> QVTPRPEAAPGARPGFRAPARIISPEIMPDNKVTFRVYSKDASKVTITGEWQTGPGGVEELVKNDTGMFSITVGPLKPELYAYNFTVDGVKALDANNV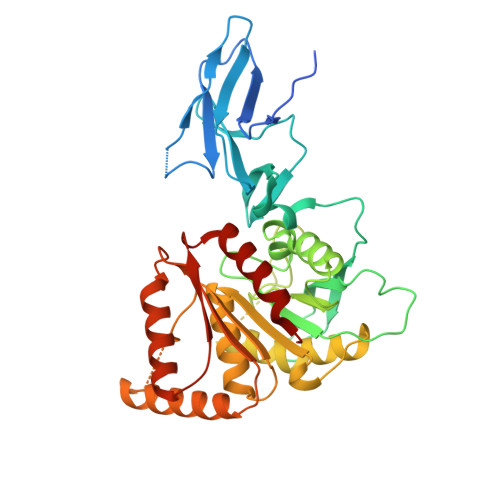QVRRDGTNYQNFFIIPGPESDLYFHKNNVPHGTVTKVWYKSSVIGFDRRMYVYTPAGYEGDTQRYPVFYLLHGAGGDEDAWTNMGRTAQIMDNLIAQGKAKPMIVVMTNGNANQAGAQNEVPPVPVTQGQQGIPSGSGMTGKFEEHLVKDVVPFIEKNFRALTGKDNRAIAGLSMGGGHTQTITNDNPGMFSYIGVFSMGIMAGRQQGGDAEKIEKERDAKIEALKKSGYKLYWIACGKDDFVYQSALTLRNTLDKHNFKYVYRESTGGHTWANWRIYLSEFAPMLFKLL>MDYGGALSAVGRELLFVTNPVVVNGSVLVPEDQCYCAGWIESRGTNGAQTASNVLQWLAAGFSILLLMFYAYQTWKSTCGWEEIYVCAIEMVKVILEFFFEFKNPSMLYLATGHRVQWLRYAEWLLTCPVILIHLSNLTGLSNDYSRRTMGLLVSDIGTIVWGATSAMATGYVKVIFFCLGLCYGANTFFHAAKAYIEGYHTVPKGRCRQVVTGMAWLFFVSWGMFPILFILGPEGFGVLSVYGSTVGHTIIDLMSKNCWGLLGHYLRVLIHEHILIHGDIRKTTKLNIGGTEIEVET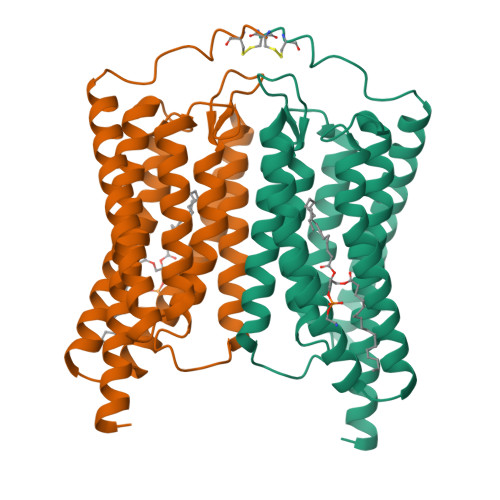LVEDEAEAGAVNKGTGK[2x]> MTRLLVLGGTTEASRLAKTLADQGFEAVFSYAGRTGAPVAQPLPTRIGGFGGVAGLVDYLTREGVSHVIDATHPFAAQMSANAVAACAQTGVALCAFERAPWTAQAGDRWTHVPDLAAAVAALPQAPARVFLAIGKQHLRDFSAAPQHHYLLRLVDPPEGPLPLPDARAVIARGPFTVQGDTELLRSETITHVVAKNAGGAGAEAKLIAARSLGLPVILIDRPAVPARDICATLEGVMGWLADHGATPRGV

In this paper we investigate the structure of the precorrin-6A reductase CobK involved in the aerobic pathway, there is a homologous enzyme CbiJ involved in the anaerobic pathway both enzymes catalyse the NADPH-dependent reduction of precorrin-6A5 to the dihydro derivative precorrin-6B6. We have determined the structure of apoenzyme, holoenzyme and a ternary complex with NADPH and product giving unprecedented insights into the structure and mechanism of CobK. CobK comprises two domains, a coenzyme binding domain and a substrate-binding domain, both of β/α architecture. CobK unusually comprises two parallel β-sheet domains arranged so the β-strands point towards the centre of the molecule where the NADPH and substrate bind.

The electron density at 1.32 Å resolution is excellent for the ternary complex with clear density for all residues, product and coenzyme with the exception of the nicotinamide of the coenzyme which is less well defined indicating its mobility. The clarity of the electron density map of the bound precorrin is remarkable. The product bound to CobK has been further modified by methylation of C5, this is a modification that can be accommodated within the active centre of the enzyme and points to the lability of the intermediate through the crystallization and data collection steps. Comparing the structure of the ternary complex with the holoenzyme reveals the ordering of the β2/ β3 loop, residues 33 to 40, across the substrate binding cleft. The propionate group on the C-ring of the tetrapyrrole appears to be important in closing this loop (an inventory of interactions involving the loop is presented in Supplementary Table S2). Note that it is the binding of product that promotes loop closure even though some of the contacts are to the coenzyme. At the active centre of CobK the coenzyme and product are held with geometry and relative orientation consistent with the hydride having been transferred from C4 of the nicotinamide to C19 of the precorrin-6B product. In the trapped product complex, the C4N of the pyridine residue of NADPH is 2.8 Å of C19 of the D-ring of the corrin macrocycle in agreement with the previously reported stereochemistry of hydride transfer. The product is almost entirely inaccessible to solvent in this time and space averaged structure and only the proprionate of the B-ring can be seen emerging from the substrate-binding pocket.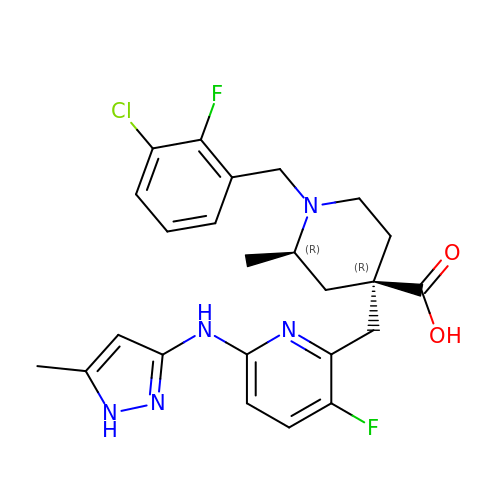(2R,4R)-1-[(3-chloro-2-fluorophenyl)methyl]-4-({3-fluoro-6-[(5-methyl-1H-pyrazol-3-yl)amino]pyridin-2-yl}methyl)-2-methylpiperidine-4-carboxylic acid | C24 H26 Cl F2 N5 O2 | YQQZZYYQTCPEAS-OYLFLEFRSA-N>SNASASSIEKGQNRVIDASLTLIRERAKLKGELVRLLGGAKASTSLLGVPLGHNSSFLQGPAFAPPRIREAIWCGSTNSATEEGKELKDPRVLTDVGDVPVQEIRDCGVDDDRLMNVISESVKLVMEEEPLRPLVLGGDHSISYPVVRAVSEKLGGPVDILHLDAHPDIYDCFEGNKYSHASSFARIMEGGYARRLLQVGIRSINQEGREQGKRFGVEQYEMRTFSKDRPMLENLKLGEGVKGVYISIDVDCLDPAFAPGVSHIEPGGLSFRDVLNILHNLQADVVGADVVEFNPQRDTVDGMTAMVAAKLVRELAAKISK[24x]

In this route, ornithine is obtained from arginine by the action of arginase (arginine amidinohydrolase, ARGAH). Similarly to other eukaryotic (Di Costanzo et al., 2010) and prokaryotic (Bewley et al., 1999) orthologues, plant ARGAHs, are binuclear manganese metalloenzymes. Together with agmatinase, formiminoglutamase, and proclavaminate aminohydrolase, ARGAHs are grouped with the Ureohydrolase Superfamily.

In this work, ARGAHs from two model plant species, A. thaliana (AtARGAH1) and Medicago truncatula (MtARGAH), are structurally characterized by X-ray crystallography and small-angle X-ray scattering (SAXS). Based on the crystal structures of AtARGAH1 and MtARGAH complexes with ornithine combined with the analysis of sequence conservation of the key residues of plant ARGAHs their dual arginase/agmatinase function in plants is discussed. A. thaliana has two ARGAH isoforms encoded by genes ARGAH1 (At4g08900) and ARGAH2 (At4g08870), which most likely appeared by gene duplication (Brownfield et al., 2008). Arabidopsis ARGAHs present dual localization; they are localized in the mitochondrial matrix (Flores et al., 2008), but they can also be targeted to plastids (Patel et al., 2017). Only ARGAH1 is actively transcribed in pollen (Brownfield et al., 2008), which likely secures the high demand of proline in pollen. The studies on ARGAH from Arabidopsis thaliana and soybean have also shown that concerted action of ARGAH and one of the arginine decarboxylases may complement the putrescine biosynthesis as the third route (Patel et al., 2017). Therefore, arginine is initially decarboxylated to agmatine and then, through the hydrolytic action of ARGAH on agmatine (agmatinase activity), putrescine is produced.> ASMEINVSKLRTDLPQVGVQPYRQVHA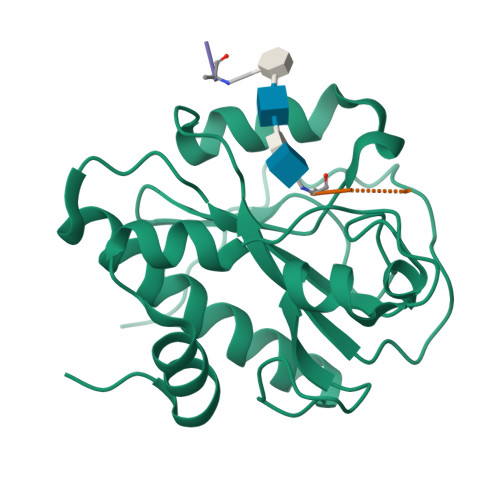HSTGNPHSTVQNEADYHWRKDPELGFFSHIVGNGAIMQVGPVDNGAWDVGGGWNAETYAAVELIESHSTKEEFMTDYRLYIELLRNLADEAGLPKTLDTGSLAGIKTAEYATNNQPNNHSDHVDPYPYLAKWGISREQFKHDIENGLTIETGWQKHHHHHH;>AEKAA[2x]> MSSAIKEVQGAPVKWVTNWTPEAIRGLVDQEKGLLDPRIYADQSLYELELERVFGRSWLLLGHESHVPETGDFLATYMGEDPVVMVRQKDKSIKVFLNQCRHRGMRICRSDAGNAKAFTCSYHGWAYDIAGKLVNVPFEKEAFCDKKEGDCGFDKAEWGPLQARVATYKGLVFANWDVQAPDLETYLGDARPYMDVMLDRTPAGTVAIGGMQKWVIPCNWKFAAEQFCSDMYHAGTTTHLSGILAGIPPEMDLSQAQIPTKGNQFRAAWGGHGSGWYVDEPGSLLAVMGPKVTQYWTEGPAAELAEQRLGHTGMPVRRMVGQHMTIFPTCSFLPGINTIRTWHPRGPNEIEVWAFTLVDADAPAEIKEEYRRHNIRNFSAGGVFEQDDGENWVEIQKGLRGYKAKSQPLNAQMGLGRSQTGHPD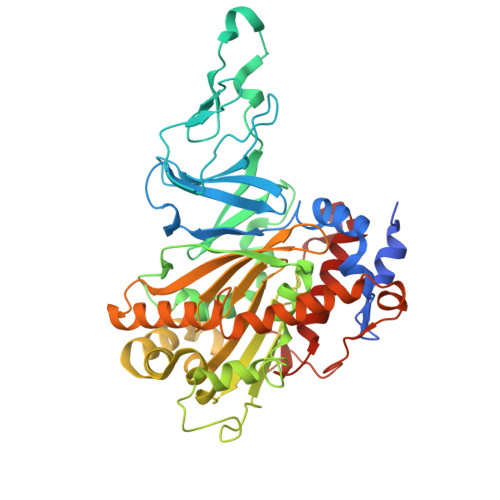FPGNVGYVYAEEAARGMYHHWMRMMSEPSWATLKP> MKKGHHHHHHGQKPKYQVRWKIIESYEGNSYTFIDPTQLPYNEKWEFPRNNLQFGKTLGAGAFGKVVEATAFGLGKEDAVLKVAVKMLKSTAHADEKEALMSELKIMSHLGQH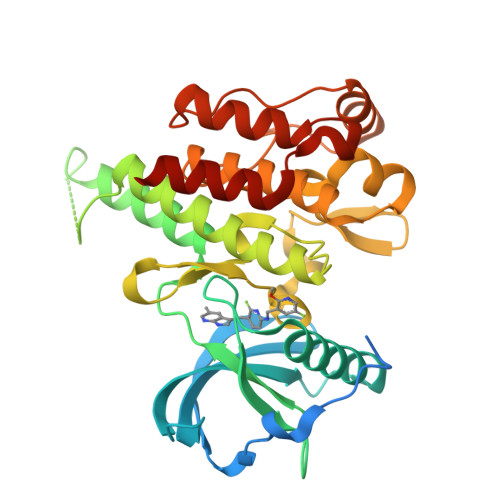ENIVNLLGACTHGGPVLVITEYCTYGDLLNFLRRKAEAMLGPSLSPGQDPEGLDKEDGRPLELRDLLHFSSQVAQGMAFLASKNCIHRDVAARNVLLTNGHVAKIGDFGLARDIMNDSNYIVKGNARLPVKWMAPESIFDSVYTVQSDVWSYGILLWEIFSLGLNPYPGILVNSKFYKLVKDGYQMAQPAFAPKNIYSIMQACWALEPTHRPTFQQITSFLQEQAQEDRR>MATLRVHPEAQAKVDVFREDLCSKTENLLGSYFPKKISELDAFLKEPALNEANLSNLKAPLDIPVPDPVKEKEKEERKKQQEKEEKEEKKKGDEDDKGPPCGPVNCNEKIVVLLQRLKPEIKDVTEQLNLVTTWLQLQIPRIEDGNNFGVAVQEKVFELMTNLHTKLEGFHTQISKYFSERG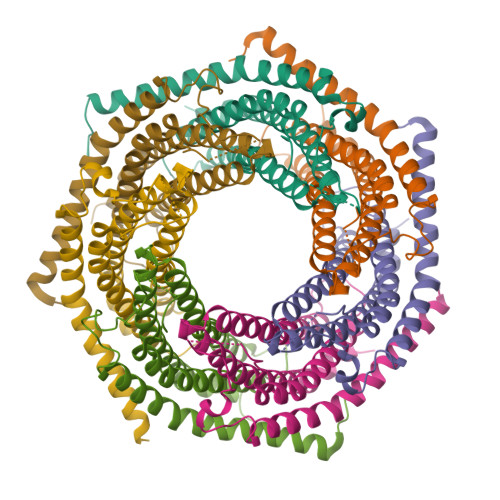DAVAKAAKQPHVGDYRQLVHELDEAEYQEIRLMVMEIRNAYAVLYDIILKNFEKLKKPRGETKGMIY[28x]[(3S)-2-oxo-2,3-dihydro-1H-indol-3-yl]acetic acid | C10 H9 N O3 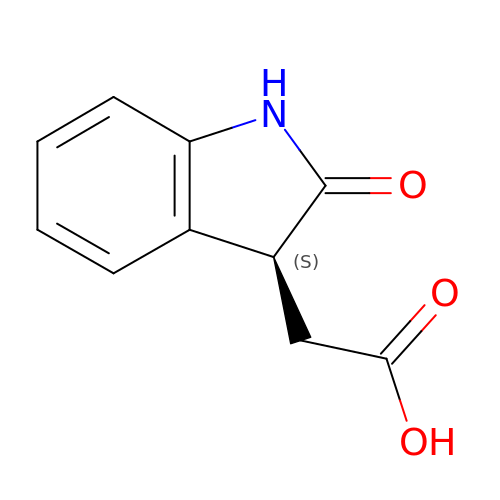| ILGMGHZPXRDCCS-ZETCQYMHSA-N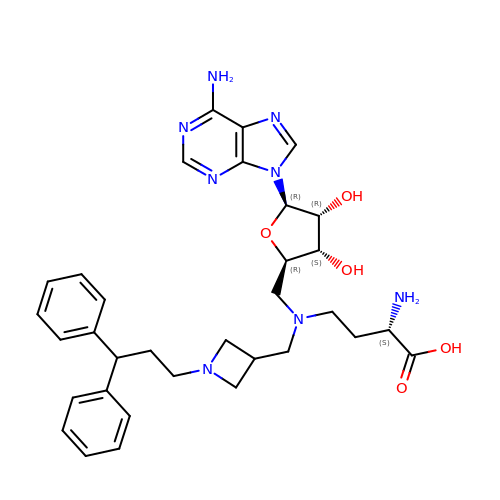5'-([(3S)-3-amino-3-carboxypropyl]{[1-(3,3-diphenylpropyl)azetidin-3-yl]methyl}amino)-5'-deoxyadenosine | C33 H42 N8 O5 | VHPRRJZGFMSHQV-JUCHKJSUSA-N> MQKRQSTKEEVYKDFQKQISDMNYYSCKAEVEVVGNKSPHNYVLIHTYKKTDNYKLEVISP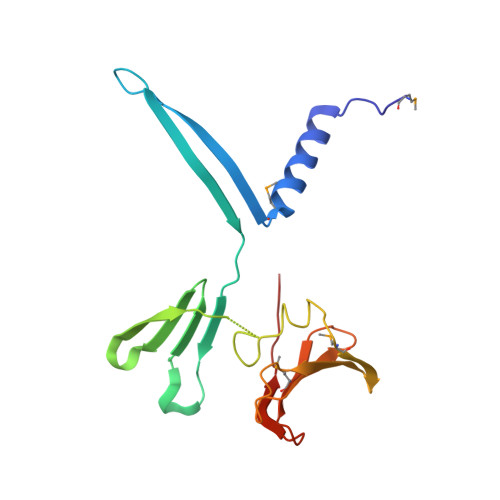KHLKGKSIEYQGDKILVKNPKISDVVELPNTGKNNQYLFVGDFIKNYLQNEEMKVKLSKGHLVLETFIPGDNKYFNKQVLYVNADTKNPEKMEVLDKEGVPRFTVKYKDFEYRN>GSHMGSASEQRVTLTNADKVLYPATGTTKSDIFDYYAGVAEVMLGHIAGRPATRKRWPNGVDQPAFFEKQLALSAPPWLSRATVAHRSGTTTYPIIDSATGLAWIAQQAALEVHVPQWRFVAEPGSGELNPGPATRLVFDLDPGEGVMMAQLAEVARAVRDLLADIGLVTFPVTSGSKGLHLYTPLDEPVSSRGA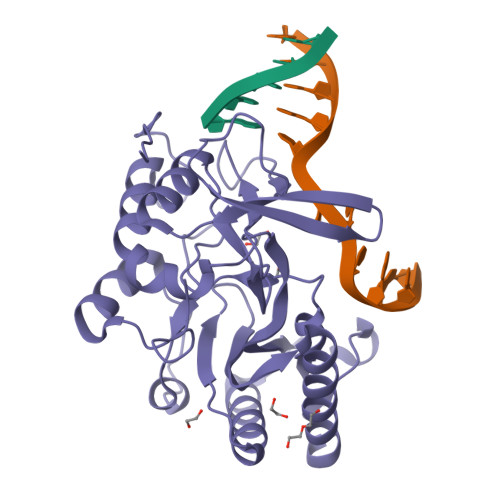TVLAKRVAQRLEQAMPALVTSTMTKSLRAGKVFVDWSQNSGSKTTIAPYSLRGRTHPTVAAPRTWAELDDPALRQLSYDEVLTRIARDGDLLERLDADAPVADRLTRY[2x]>GHMKQSHFFAHLSRLKLINRWPLMRNVRTENVSEHSLQVAMVAHALAAIKNRKFGGNVNAERIALLAMYHDASAVLTGDLPTPVKYFNSQIAQEYKAIEKIAQQKLVDMVPEELRDIFAPLIDEHAYSDEE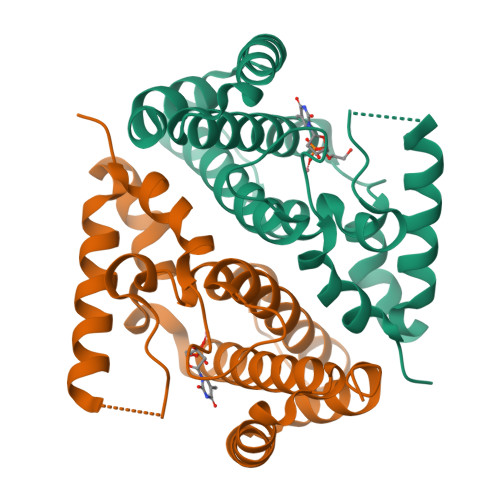KSLVKQADALCAYLKCLEELAAGNNEFLLAKTRLEATLEARRSQEMDYFMEIFVPSFHLSLDEISQDSPL[2x]>STAGKVIKCKAAVLWEEKKPFSIEEVEVAPPKAHEVRIKMVATGICRSDDHVVSGTFVTPLPVIAGHEAAGIVESIGEGVTTVRPGDKVIPLFTPQCGKCRVCKHPEGNFCLKNDLSMPRGTMQDGTSRFTCRGKPIHHFLGTSTFSQYTVVDEISVAKIDAASPLEKVCLIGCGFSTGYGSAVKVAKVTQGSTCAVFGLGGVGLSVIMGCKAAGAARIIGVDINKDKFAKAKEVGATECVNPQDYKKPIQEVLTEMSNGGVDFSFEVIGRLDTMVTALSCCQEAYGVSVIVGVPPDSQNLSMNPMLL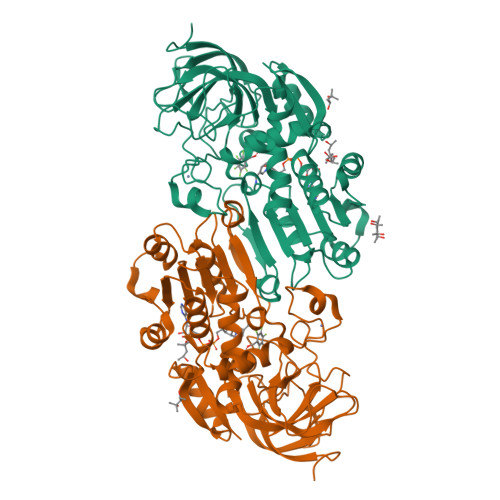LSGRTWKGAIFGGFKSKDSVPKLVADFMAKKFALDPLITHVLPFEKINEGFDLLRSGESIRTILTF[2x]> XCELC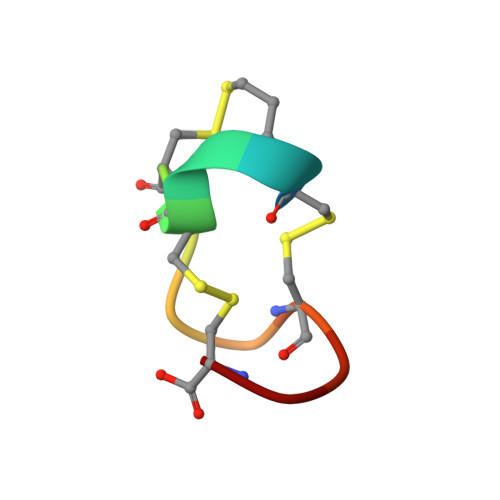CNPLCAGC> NKGSIEGREPAVYFKEQFLDGDGWTSRWIESKHKSDFGKFVLSSGKFYGDEEKDKGLQTSQDARFYALSASFEPFSNKGQTLVVQFTVKHEQNIDCGGGYVKLFPNSLDQTDMHGDSEYNIMFGPDICGPGTKKVHVIFNYKGKNVLINKDIRCKDDEFTHLYTLIVRPDNTYEVKIDNSQVESGSLEDDWDFLPGSGDPSIYAYD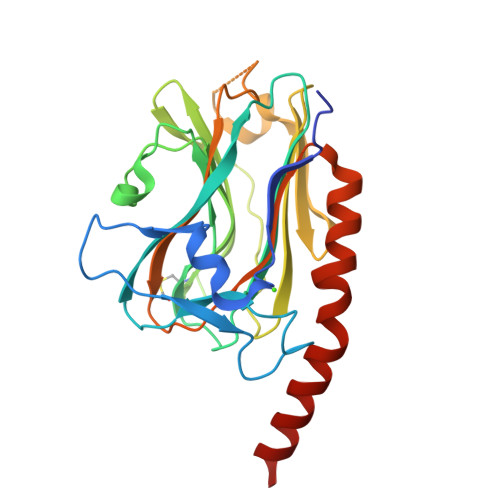NFGVLGLDLWQVKSGTIFDNFLITNDEAYAEEFGNETWGVTKAAEKQMKDKQDEEQRLK6-phenyl-1-(pyridin-4-ylmethyl)-1H-pyrazolo[3,4-b]pyridine-4-carboxylic 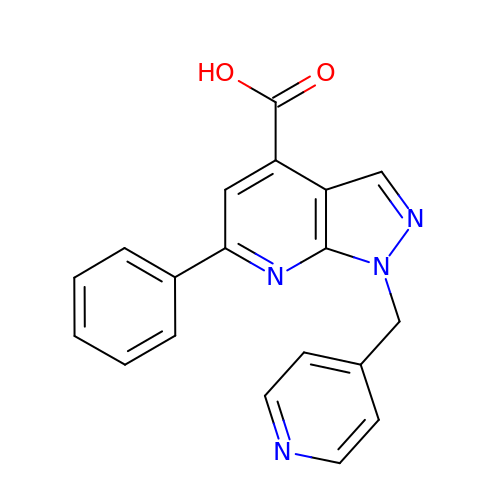acid | C19 H14 N4 O2 | KCTGBSZXRNRGOD-UHFFFAOYSA-N> GDTETAIDNAIARVADTVASGPSNSTSIPALTAVETGHTSQVEPSDTMQTRHVKNYHSRSESTVENFLSRSACVYIEEYYTKDQDNVNRYMSWTINARRMVQL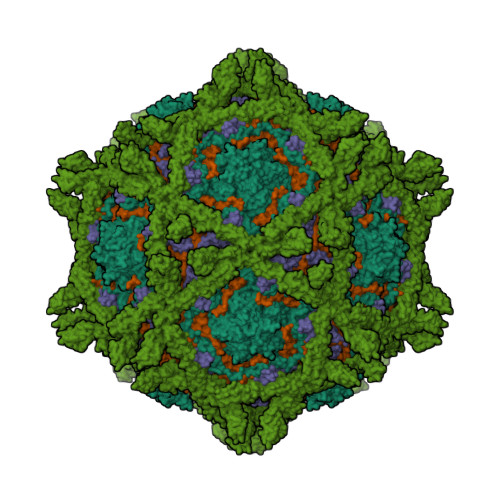RRKFELFTYMRFDMEITFVITSRQLPGTSIAQDMPPLTHQIMYIPPGGPVPNSVTDFAWQTSTNPSIFWTEGNAPPRMSIPFISIGNAYSNFYDGWSHFSQNGVYGYNALNNMGKLYARHVNKDTPYQMSSTIRVYFKPKHIRVWVPRPPRLSPYIKSSNVNFNPTNLTDERSSITYVPDTIRPDVRTN;> GLPVLNTPGSNQFMTSDDFQSPSAMPQFDVTPHMDIPGEVHNLMEIAEVDSVVPVNNIKANLQSMDAYHIEVNTGNYQGEKIFAFQMQPGLESVFKRTLMGEILNYYAHWSGSIKLTFTFCGSAMATGKLLLAYSPPGADVPATRKQAMLGTHMIWDIGLQSSCVLCIPWISQTHYRLVQQDEYTSAGNVTCWYQTGIVVPPGTPNKCVVLCFASACNDFSVRMLRDTPFIGQTALLQ;> PSAEECGYSDRVRSLTLGNSTITTQESANVVVGYGRWPEYLRDDEATAEDQPTQPDVATCRFYTLESVQWEKNSAGWWWKFPEALKDMGLFGQNMLYHYLGRAGYTIHVQCNASKFHQGCLLVVCVPEAEMGCSQTDKEVAAMNLTKGEAAHKFEPTKTNGEHTVQSIVCNAGMGVGVGNLTIYPHQWINLRTNNCATIVMPYVNSVPMDNMFRHYNFTLMVIPFAPLDYAAQASEYVPVTVTIAPMCAEYNGLRLAYQQ;> MGAQVSTQKTGAHETGLNASGNSIIHYTNINYYKDAASNSANRQDFTQDPGKFTEPVKDIMIKTMPALNS;> MTVARPSVPAALPLLGELPRLLLLVLLCLPAVWQDCGLPPDVPNAQPALEGRTSFPEDTVITYKCEESFVKIPGEKDSVICLKGSQWSDIEEFCNRSCEVPTRLNSASLKQPYITQNYFPVGTVVEYECRPGYRREPSLSPKLTCLQNLKWSTAVEFCKKKSCPNPGEIRNGQIDVPGGILFGATISFSCNTGYKLFGSTSSFCLISGSSVQWSDPLPECREIYCPAPPQIDNGIIQGERDHYGYRQSVTYACNKGFTMIGEHSIYCTVNNDEGEWSGPPPECRGKSLTSKVPPTVQKPTTVNVPTTEVSPTSQKTTTKTTTPNAQATRSTPVSRTTKHFHETTPNKGSGTTSGTTRLLSGHTCFTLTGLLGTLVTMGLLT Efficient γ-herpesvirus lytic phase replication requires a virally encoded UNG-type uracil-DNA glycosylase as a structural element of the viral replisome. Uniquely, γ-herpesvirus UNGs carry a seven or eight residue insertion of variable sequence in the otherwise highly conserved minor-groove DNA binding loop. The UNG leucine loop is a conserved structural feature which is responsible for widening the DNA minor groove and flipping pyrimidines out of the base stack and, in the case of uracil, into the UNG active site for catalysis. kUNG, in common with other known UNGs, comprises a single C-terminal globular domain made up of a four-stranded parallel β-sheet flanked by six α-helices, with an additional left-handed coil of three helices at the N-terminus.

The crystal structures reveal that upon DNA binding, the loop extension favours the disc-like configuration previously observed in the EBV UNG–Ugi complex. In the kUNG–dsDNA structure, the kUNG leucine loop extension (residues G222-R229) is ordered via a hydrogen bonding network centred on the side-chain of Q212. In the kUNG–dsDNA structure reported here, the orphan base of nucleotide dA27 is actively flipped out of the DNA duplex by the extended segment (common to all γ-herpesvirus UNGs) of the leucine loop, a feature not seen in any of the previously published structures of UNG–dsDNA complexes from human, Deinococcus radiodurans, Thermus thermophilus and Vaccinia virus. The extrahelical conformation of nucleotide dA27 is conserved in all four monomers of the crystal asymmetric unit where the base is solvent exposed and forms no contacts with neighboring molecules. Hydrogen bonds between the NH2 of the adenine base in dA27 and the phosphate of the neighboring nucleotide, dT26 rigidifies the orphan base in the crystal providing clear electron density. Indeed, this fact is exploited in UNG activity assays which rely on the fluorescence increase upon liberation from the base stack of 2-aminopurine bases in the orphan position. In the kUNG–dsDNA structure however, both the adenine base and the deoxyribose moiety of dA27 are significantly displaced from the duplex stack with a distorted backbone conformation being stabilised by hydrogen bonding between the guanidinium head group of R223 in kUNG and the phosphate moiety of dA27 (see Supplementary Table S1 for a summary of protein–DNA contacts). The position in the base stack usually occupied by dA27 is taken up by L220 of kUNG in a manner strikingly similar to that of the strictly conserved ‘doorstop’ leucine L217 which displaces the substrate uracil base from the DNA helix flipping it into the UNG active site. In contrast, nine residues of kUNG (S215-R223), including the entirety of a five-residue helix (P216-L220), intercalate between the DNA bases presenting two leucine sidechains to flip out both the substrate deoxyuridine and its partner nucleotide in a duplex nucleotide-flipping mechanism.

>SASGVDDRDLLLAPKWISFLSLSSFLKQKLLSLLRQIRELRLTTTVYPPQDKLMWWSHCCDPEDIKVVILGQDPYHKGQATGLAFSVDPQCQVPPSLRSIFRELEASVPNFSTPSHGCLDSWARQGVLLLNTVLTVEKGRAGSHEGLGWDWFTSFIISSISSKLEHCVFLLWGRKAIDRTPLINAQKHLVLTAQHPSPLASLGGRHSRWPRFQGCNHFNLANDYLTRHRRETVDWGLLEQ[4x]>DSISLSLINEGPSYASKVSVGSNKQQQTVIIDTGSSDFWVVDSNAQCGKGVDCKSSGTFTPSSSSSYKNLGAAFTIRYGDGSTSQGTWGKDTVTINGVSITGQQIADVTQTSVDQGILGIGYTSNEAVYDTSGRQTTPNYDNVPVTLKKQGKIRTNAYSLYLNSPSAETGTIIFGGVDNAKYSGKLVAEQVTSSQALTISLASVNLKGSSFSFGDGALLDSGTTLTYFPSDFAAQLADKAGARLVQVARDQYLYFIDCNTDTSGTTVFNFGNG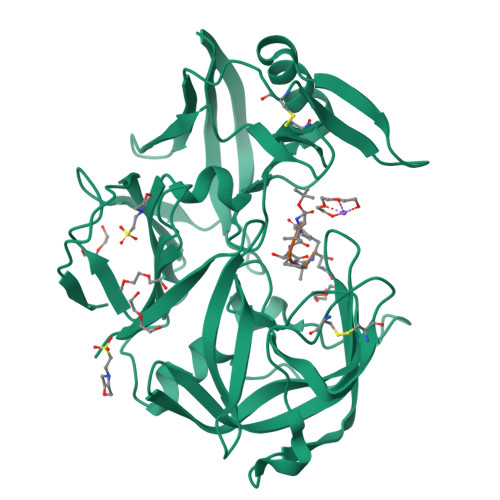AKITVPNTEYVYQNGDGTCLWGIQPSDDTILGDNFLRHAYLLYNLDANTISIAQVKYTTDSSISAV[4x];>[4x]XVVFAFA> SALRLQMLGTGGAFAKKYFNNNALLYAGDFTLLIDCGITAPLALHTIGKSVEEIDAVLITHIHGDHVGGLEELAFRRKFGSGRKPILYIAENLVEPLWENTLKGGLSQDGVIHSLNDVFDVRLLKESEPAQL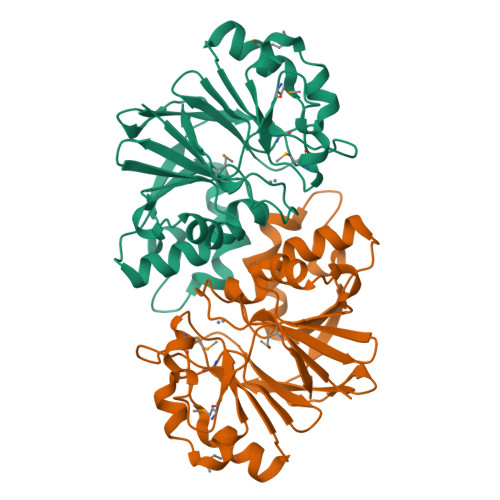APELKVELIRTPHIPGKPSYSLYINDEIFYSADMTFEPELLMRLVRERGCRRIFHEVQLTGKGEVHTTLQELLSLPTEIQSQILLKHYSDDMESFRGATGNMDFLRQHEVYTL N-(4-chlorophenyl)-2-[(pyridin-4-ylmethyl)amino]benzamide | C19 H16 Cl N3 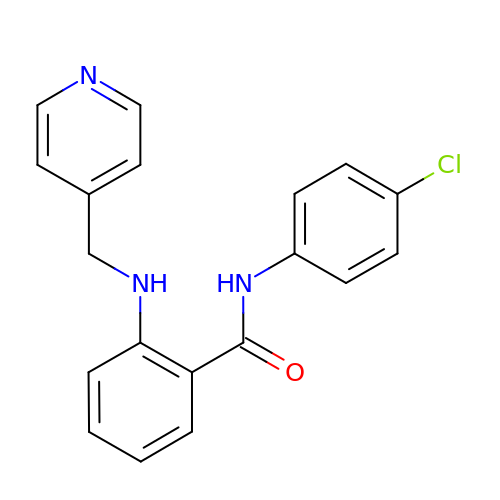O | GGPZCOONYBPZEW-UHFFFAOYSA-N>MGSTGNAEIQIIPTHSSDEEANLFAMQLASAAVLPMALKAAIELDVLEIMAKSVPPSGYISPAEIAAQLPTTNPEAPVMLDRVLRLLASYSVVTYTLRELPSGKVERLYGLAPVCKFLTKNEDGVSLAPFLLLATDKVLLEPWFYLKDAILEGGIPFNKAYGMNIFDYHGTDHRINKVFNKGMSSNSTITMKKILEMYNGFEGLTTIVDVGGGTGAVASMIVAKYPSINAINFDLPHVIQDAPAFSGVEHLGGDMFDGVPKGDAIFIKWICHDWSDEHCLKLLKNCYAALPDHGKVIVAEYILPPSPDPSIATKVVIHTDALMLAYNPGGKERTEKEFQALAMASGFRGFKVASCAFNTYVME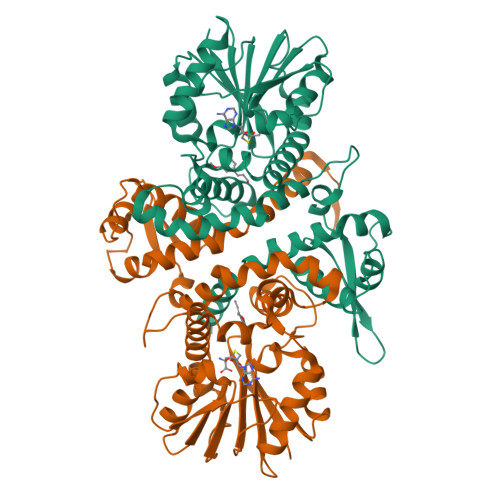FLKTA[4x]> MAWPKVQPEVNIGVVGHVAHGKTTLVQAITGIWTSKHSEELKRGMTIKLGYAETNIGVCESCKKPEAYVTEPSCKSCGSDDEPKFLRRISFIDAPGHEVLMATMLSGAALMDGAILVVAANEPFPQPQTREHFVALGIIGVKNLIIVQNKVDVVSKEEALSQYRQIKQFTKGTWAENVPIIPVSALHKINIDSLIEGIEEYIKTPYRDLSQKPVMLVIRSFDVNKPGTQFNELKGGVIGGSIIQGLFKVDQEIKVLPGLRVEKQGKVSYEPIFTKISSIRFGDEEFKEAKPGGLVAIGTYLDPSLTKADNLLGSIITLADAEVPVLWNIRIKYNLLERVVGAKEMLKVDPIRAKETLMLSVGSSTTLGIVTSVKKDEIEVELRRPVAVWSNNIRTVISRQIAGRWRMIGWGLVEI

In eukaryotic and archaeal cells, the initiator tRNA carrier is the e/aIF2 heterotrimer. In its GTP-bound form, this factor specifically binds Met-tRNAiMet and brings it to the initiation complex. The γ subunit forms the core of the heterotrimer and contains the GTP-binding pocket. α and β are bound to γ but do not interact together. We were able to observe GTP hydrolysis by aIF2 or by its isolated γ subunit.

H97A and D19A mutants were crystallized in the same conditions as those used for wt-aIF2γ but in the presence of GTP-Mg2+. In keeping with the observed decreased rates of GTP hydrolysis, we observed that GTP was intact within the crystals grown at 4°C. In the D19A-GTP4 and H97A-GTP4 structures, GTP is tightly bound to the canonical nucleotide-binding pocket in a position similar to that of GDPNP in wt-aIF2γ. If D19 is mutated to alanine (D19A-GTP4 structure), the second magnesium is not observed in keeping with the involvement of D19 in Mg2 coordination. One water molecule is still bound to G44 and to the β and γ phosphates of GTP. The catalytic H97 is in the non-activated conformation and GTP is intact. Without these, the ion would be unstable at this position, as it is shown by its absence in the crystal structure of the D19A mutant.>MTTLTRQDLNFGQVVADVLCEFLEVAVHLILYVREVYPVGIFQKRKKYNVPVQMSCHPELNQYIQDTLHCVKPLLEKN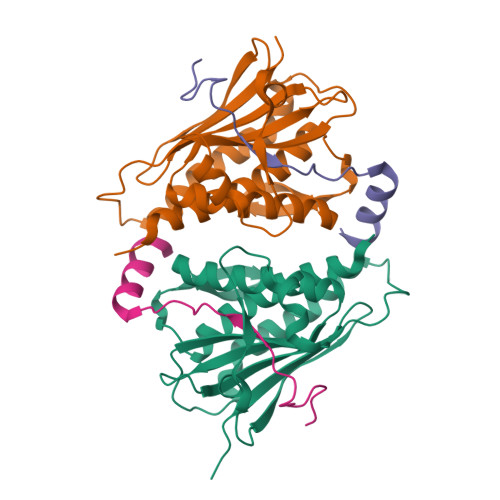DVEKVVVVILDKEHRPVEKFVFEITQPPLLSISSDSLLSHVEQLLAAFILKISVCDAVLDHNPPGCTFTVLVHTREAATRNMEKIQVIKDFPWILADEQDVHMHDPRLIPLKTMTSDILKMQLYVEERAHKGS[2x];>[2x]RFIPWFPYDGSKLPLRPKRSPPVISEEAAEDVKQYLT>MVLAGLLLLLTLLAGAHLLWGRWKLRNLHLPPLVPGFLHLLQPNLPIHLLSLTQKLGPVYRLRLGLQEVVVLNSKRTIEEAMIRKWVDFAGRPQIPSYKLVSQRCQDISLGDYSLLWKAHKKLTRSALLLGTRSSMEPWVDQLTQEFCERMRVQAGAPVTIQKEFSLLTCSIICYLTFGNKEDTLVHAFHDCVQDLMKTWDHWSIQILDMVPFLRFFPNPGLWRLKQAIENRDHMVEKQLRRHKESMVAGQWRDMTDYMLQGVGRQRVEEGPGQLLEGHVHMSVVDLFIGGTETTASTLSWAVAFLLHHPEIQRRLQEELDRELGPGASCSRVTYKDRARLPLLNAT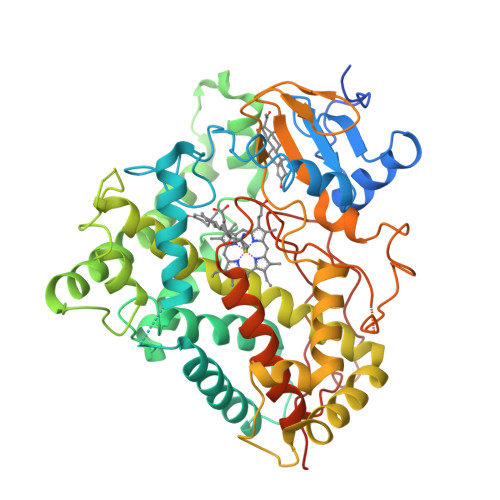IAEVLRLRPVVPLALPHRTTRPSSIFGYDIPEGMVVIPNLQGAHLDETVWEQPHEFRPDRFLEPGANPSALAFGCGARVCLGESLARLELFVVLARLLQAFTLLPPPVGALPSLQPDPYCGVNLKVQPFQVRLQPRGVEAGAWESASAQ[4x]>MGIVCHTTATSPISAVTCPPGENLCYRKMWCDVFCSSRGKVVELGCAATCPSKKPYEEVTCCSTDKCNPHPKQRPG[4x];>WRYYESSLLPYPD[4x]

Three-finger proteins (TFPs) are a class of proteins (peptides) including TFNs and their mammalian homologue that show similar three-finger structure as TFNs. The three-finger neurotoxins (TFNs) are a collection of such toxin peptides used by the snake to kill the prey through binding and blocking ion channels in the neurological system. The α-neurotoxin binds to and block the muscle type nicotinic acetylcholine receptor (α12β1γ(ε)δ nAChR) on the neuromuscular junction, leading to paralysis of the prey. We introduce a working pipeline for expression, purification and validation of disulfide-bond rich three-finger proteins using E. coli as the expression host.

We previously reported the production of bioactive recombinant α-Bungarotoxin (rec-αBtx), in which we used radioimmunoassay to determine the optimal refolding conditions. To test the binding specificities of the rTFPs, HAP peptide, a known peptide derived from the nicotinic acetylcholine receptor, was mixed with various rTFPs and separated on a 15% native PAGE gel at pH 5.0. HAP peptide was only able to shift rec-αBtx and only slightly shift rec-Hannalgesin, but not rec-MTα, rec-mPate B, rec-κBtx, rec-Mambalgin-1 and rec-hSlurp1. We compared the elution volume of rec-αBtx, rec-κBtx, rec-mPate B in gel filtration column (Superdex 75 10 300 GL, GE Healthcare), and found that rec-αBtx, which were known as a monomer, eluted much later than rec-κBtx, suggesting rec-κBtx was not a monomer, which is in accordance with earlier reports that κBtx exists in dimeric form and also with the solved crystal structures, while rec-mPate B elute at similar volume as rec-κBtx, suggesting rec-mPate B was also a dimmer. Six rTFPs’ structures were solved with x-ray crystal diffraction data using molecular replacement with known homologous structures. From the structural alignment of the solved structures with their native counterparts (such as rec-aBtx-HAP complex, rec-αCTX, rec-kBtx, rec-mambalgin) or with their most homologous native counterparts (such as rec-Hannalgesin and rec-MTα, whose crystal structures were not reported, known homologous TFPs with known structure, such as αCTX and MT1, respectively, were used as the alignment counterpart). Through extensive biochemical assays and structural analysis, we showed that our rTFPs were almost identical to their native counterparts. Though it was generally considered very difficult to obtain rTFPs using either E. coli or other expression systems, with our pipeline, we could repeatedly obtain over one hundred mg of rec-MTα, rec-Hannalgesin, rec-αCTX and rec-mPate B, tens of milligrams of rec-mambalgin-1, Slurp1 and milligrams of rec-kBtx and rec-αBtx through one round of experiment (usually finished within 4 ~ 5 weeks).Dynein is activated for long-distance processive movement along microtubules through interactions with its general cofactor, dynactin, and one of many so-called “activating adaptors”. The activating adaptors (hereafter referred to as adaptors) fulfill multiple roles; they mediate key interactions that stabilize the dynein–dynactin complex, recruit cargoes, and regulate dynein’s activity and processive motility. Here, we structurally and biochemically characterize the interactions of LIC1 with two adaptors, BICD2 and CRACR2a. Crystallographic analysis shows that the LIC1–adaptor interaction has a conserved hydrophobic character, with the amphipathic LIC1 helix displaying a nearly identical conformation and its hydrophobic face embedded in a hydrophobic cleft in the three adaptor subfamilies.

A crystal structure of CRACR2a47–122 (MBP removed) in complex with LIC1433–458 was obtained at 2.66 Å resolution. The monoclinic crystals, belonging to space group P21, contain eight complexes in the asymmetric unit. The two EF-hands of CRACR2a display a canonical fold, consisting of incoming helix (helices α1 and α3), loop and exiting helix (helices α2 and α4). As indicated by the ITC titration, the structure reveals a single Ca2+-binding site. Consistent with the sequence analysis, the Ca2+ density is observed within the second EF-hand domain of all the complexes of the asymmetric unit, whereas none of the complexes displays Ca2+ density within the first EF-hand. In CRACR2a, Ca2+ is ligated by the side chains of D97, D99, N101, E108, the main-chain carbonyl oxygen of Y103 and a water molecule that is in turn coordinated by T105. Like in other members of the EF-hand family, the target-binding site consists of a hydrophobic cleft formed between the incoming and exiting helices of the two EF-hand domains. The hydrophobic face of the LIC1 helix binds in this cleft, and the same conformation is observed in all eight complexes of the asymmetric unit. Like in the complexes with the HOOK domain18 and BICD2, highly conserved, hydrophobic residues of the LIC1 helix (L444, F447, F448, and L451) insert into the hydrophobic cleft formed by the EF-hand pair of CRACR2a. We have shown here that CRACR2a is regulated by Ca2+ binding to a single site within the EF-hand pair, which in turn triggers the binding of the LIC1 helix.

>[8x]GGQLVMLRKAQEFFQTCDAEGKGFIARKDMQRLHKELPLSLEELEDVFDALDADGNGYLTPQEFTTGFSHFFFSQN;>NMKAGATSEGVLANFFNSLLSKKTG[8x]> GPLGSMTQNNAPESVAAEGTVAGQQTDTTKPEPSSQPAPEPPSQVTTDFPPNNKPNDVPATEPASSSPRPTEPPAPPPPKPTIALSPLDIATLTFPDGTRGTFPAPPQTSAQSVSTPSIASGHVTPQRDTDTASITSVAGTLRGVTGTAGDLASLLAGDGLGRKSKAWRVLRAQQQACGEGSGEEGEITEIEGLGLGEGMEGFERELDNIPDTLPDDERLALWKGKLKHYLILSSAGKPIWSRHGDLSLVNSTMGVVQTIISFYEGARNPLLGFTAGKVRFVILIKGPLYFVAISRLRESDAQLRAQLEALYMQILSTLTLPILTNIFAHRPSTDLRGPLQGTESLLASLADSFTKGSPSTLLSALECLRLRKSQRQAITNIFLKSRCEELLYGLLVAGGKLVSVIRPRKHSLHPSDLQLI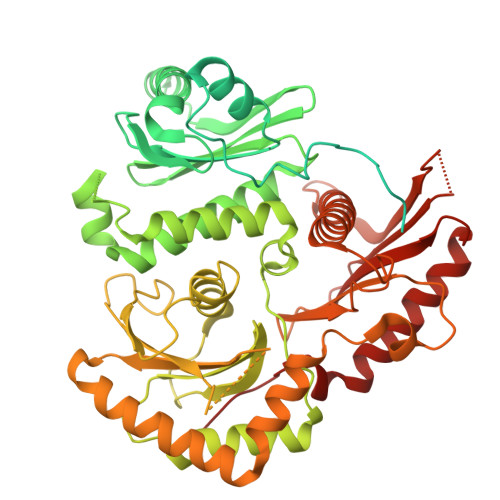FNMLFESGGIKGNGGENWIPLCLPAFNNTGYLYMYVSFLDDKAPDDQNQPPESSNLDASNKNSSNTPDDDLTALILISPSREAFYALQSMRTRLVSQLLSTGYLSLIRSTALSGRPSITSILPKTPLLHFLYKSRPNVQWCMSSLSSLTPPGATATETLLARRKLMSVYEELHAALHARHAHLRVVYSTADEKEGEGLACLGWSTPAFEVYCVAPGCVGRAGMAREVNRVVQWARREEERLFILGGGVF> MGATTPSANQNWRLLRDESAQLRIADVLQRKEQFRPLAKRSFIFPASPQAVWLQVQLPAQKVPSWLWIFAPRVQYLDYYLVQDGQLVRDQHTGESRPFQERPL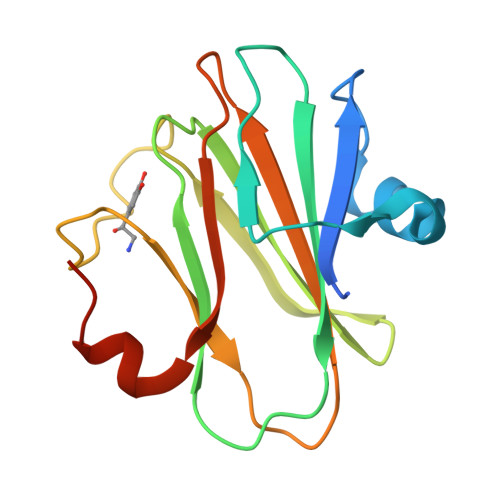PSRSYLFSLPVDGKPMTLYVRMTSNHPLMAWFDQIDEAGLVGLEHHHHHH>MQAATVVINRRALRHNLQRLRELAPASKMVAVVKANAYGHGLLETARTLPDADAFGVARLEEALRLRAGGITKPVLLLEGFFDARDLPTISAQHFHTAVHNEEQLAALEEASLDEPVTVWMKLDTGMHRLGVRPEQAEAFYHRLTQCKNVRQPVNIVSHFARADEPKCGATEKQLAIFNTFCEGKPGQRSIAASGGILLWPQSHFDWVRPGIILYGVSPLEDRSTGADFGCQPVMSL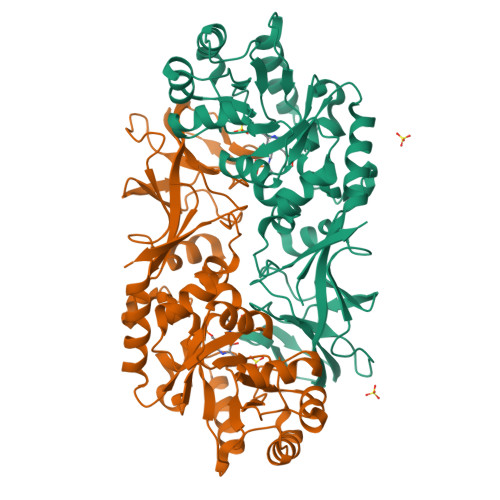TSSLIAVREHKAGEPVGYGGTWVSERDTRLGVVAMGFGDGYPRAAPSGTPVLVNGREVPIVGRVAMDMICVDLGPQAQDKAGDPVILWGEGLPVERIAEMTKVSAYELITRLTSRVAMKYVD[4x]> GSHMTRETERFPAREFQRDLLDWFARERRDLPWRKDRDPYKVWVSEVMLQQTRVETVIPYFEQFIDRFPTLEALADADEDEVLKAWEGLGYYSRVRNLHAAVKEVKTRYGGKVPDDPDEFSRLKGVGPYTVGAVLSLAYGVPEPAVNGNVMRVLSRLFLVTDDIAKCSTRKRFEQIVREIMAYENPGAFNEALIELGALVCTPRRPSCLLCPVQAYCQAFAEGVAEELPVKMKKTAVKQVPLAVAVLADDEGRVLIRKRDSTGLLANLWEFPSCETDGADGKEKLEQMVGEQYGLQVELTEPIVSFEHAFSHLVWQLTVFPGRLVHGGPVEEPYRLAPEDELKAYAFPVSHQRVW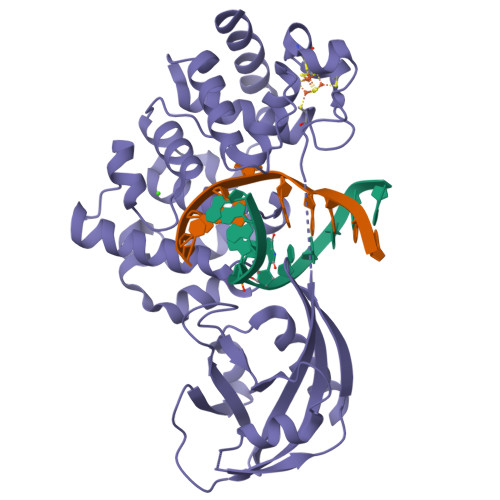REYKEWASGVRPPP> DWVEQLILAGSSLRSVFATSKEFDGPCQNEIDLLFSECNDEIDNAKLIMKERRFTASYTFAKFSTGSMLLTKDIVGKSGVSIKRLPTELQRKFLFDDVYLDKEIEKVTIEARKSNPYPQISESSLLFKDALDYMEKTSSDYNLWKLSSILFDPVSYPYKTDNDQVKMALLKKERHCRLTSWIVSQIGPEIEEKIRN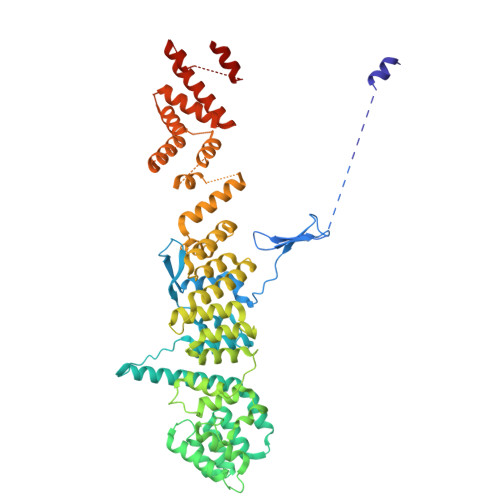SSNEIEQIFLYLLLNDVVRASKLAIESKNGHLSVLISYLGSNDPRIRDLAELQLQKWSTGGCSIDKNISKIYKLLSGSPFEGLFSLKELESEFSWLCLLNLTLCYGQIDEYSLESLVQSHLDKFSLPYDDPIGVIFQLYAANENTEKLYKEVRQRTNALDVQFCWYLIQTLRFNGTRVFSKETSDEATFAFAAQLEFAQLHGHSLFVSCFLNDDKAAEDTIKRLVMREITLLRASTNDHILNRLKIPSQLIFNAQALKDRYEGNYLSEVQNLLLGSSYDLAEMAIVTSLGPRLLLSNNPVQNNELKTLREILNEFPDSERDKWSVSINVFEVYLKLVLDNVETQETIDSLISGMKIFYDQYKHCREVAACCNVMSQEIVSKILEKNNPSIGDSKAKLLELPLGQPEKAYLRGEFAQDLMKCTYKI> GGTGGGGCACGCCCCACC

Nine new crystal structures of CG-rich DNA 18-mers with the sequence 5′-GGTGGGGGC-XZ-GCCCCACC-3′, which are related to the bacterial repetitive extragenic palindromes, are reported. All 18-mers crystallized as isomorphic tetragonal crystals with one strand of a right-handed antiparallel duplex in the asymmetric unit. All reported structures co-crystallized with the Sr2+ cation located between nucleotides 6 and 7 and (by symmetry) 12 and 13.

Two of the four YR and RY variants unable to form Watson–Crick pairs were crystallized, Chom-18-AC and Chom-18-GT, but their base-pairing topology was not assigned. Only Chom-18-CG, Chom-18-GC and Chom-18-AC have all dinucleotides assigned (classified as NtC classes AA##); unassigned dinucleotides (NtC class NANT) are mostly localized near the central base pair. When we measure the distances between the C1′ atom of nucleotide 9 and C1′ of its symmetry-related base-paired nucleotide 10 in all 18-mers, the order from the shortest to the longest is TT (7.9 Å) < CC < TC < GT < GC < AC < AT < TA < CG < AG (12.1 Å).>MSQHNEKNPHQHQSPLHDSSEAKPGMDSLAPEDGSHRPAAEPTPPGAQPTAPGSLKAPDTRNEKLNSLEDVRKGSENYALTTNQGVRIADDQNSLRAGSRGPTLLEDFILREKITHFDHERIPERIVHARGSAAHGYFQPYKSLSDITKADFLSDPNKITPVFVRFSTVQGGAGSADTVRNIRGFATKFYTEEGIFDLVGNNTPIFFIQDAHKFPDFVHAVKPEPHWAIPQGQSAHDTFWDYVSLQPETLHNVMWAMSDRGIPRSYRTMEGFGIHTFRLINAEGKATFVRFHWKPLAGKASLVWDEAQKLTGRDPDFHRRELWEAIEAGDFPEYELGFQLIPEEDEFKFDFDLLDPTKLIPEELVPVQRVGKMVLNRNPDNFFAENEQAAFHPGHIVPGLDFTNDPLLQGRLFSYTDTQISRLGGPNFHEIPINRPTCPYHNFQRDGMHRMGIDTNPANYEPNSINDNWPRETPPGPKRGGFESYQERVEGNKVRERSPSFGEYYSHPRLFWLSQTPFEQRHIVDGFSFELSKVVRP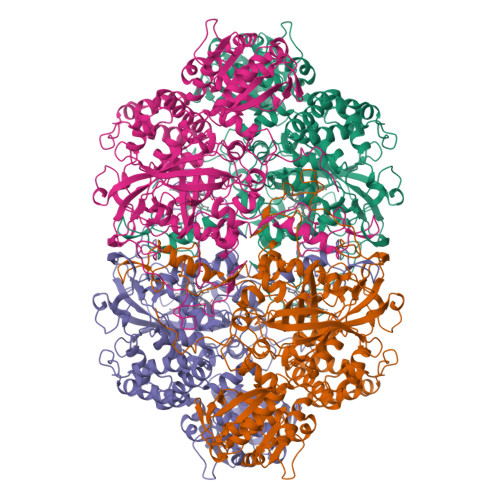YIRERVVDQLAHIDLTLAQAVAKNLGIELTDDQLNITPPPDVNGLKKDPSLSLYAIPDGDVKGRVVAILLNDEVRSADLLAILKALKAKGVHAKLLYSRMGEVTADDGTVLPIAATFAGAPSLTVDAVIVPCGNIADIADNGDANYYLMEAYKHLKPIALAGDARKFKATIKIADQGEEGIVEADSADGSFMDELLTLMAAHRVWSRIPKIDKIPA[4x]> MANVNKTPGKTRRAEVAGGGFAGLTAAIALKQNGWDVRLHEKSSELRAFGAGIYLWHNGLRVLEGLGALDDVLQGSHTPPTYETWMHNKSVSKETFNGLPWRIMTRSHLHDALVNRARALGVDISVNSEAVAADPVGRLTLQTGEVLEADLIVGADGVGSKVRDSIGFKQDRWVSKDGLIRLIVPRMKKELGHGEWDNTIDMWNFWPRVQRILYSPCNENELYLGLMAPAADPRGSSVPIDLEVWVEMFPFLEPCLIEAAKLKTARYDKFETTKLDSWTRGKVALVGDAAHAMCPALAQGAGCAMVNAFSLSQDLEEGSSVEDALVAWETRIRPIT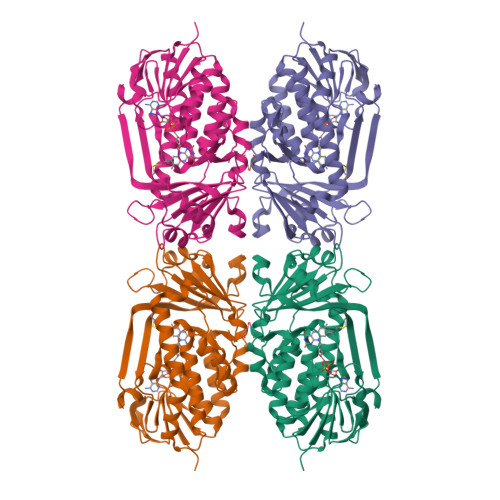DRCQALSGDYAANRSLSKGNMFTPAALEAARYDPLRRVYSWPQ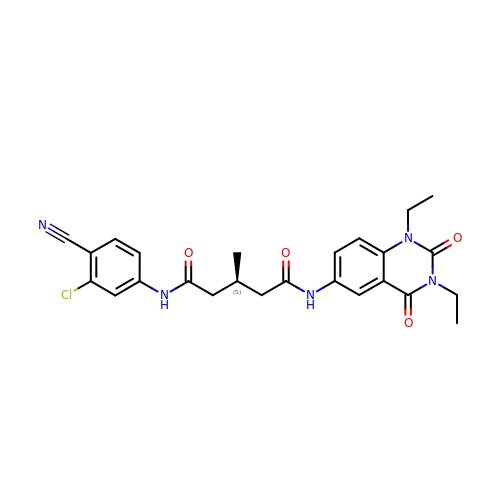(3S)-N~1~-(3-chloro-4-cyanophenyl)-N~5~-(1,3-diethyl-2,4-dioxo-1,2,3,4-tetrahydroquinazolin-6-yl)-3-methylpentanediamide | C25 H26 Cl N5 O4 | BOZDOTVXHRNQKE-HNNXBMFYSA-N> MGSS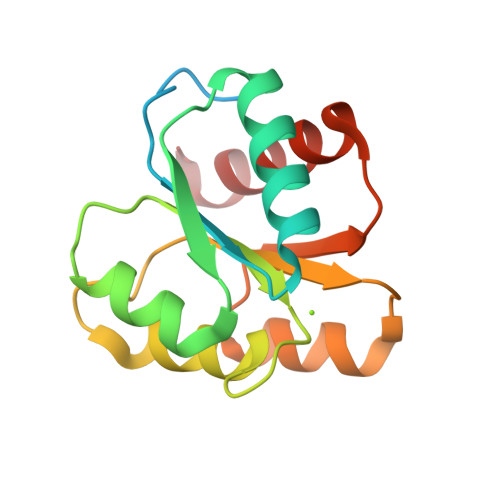HHHHHHSSGPQQGLRENLYFQGMADKELKFLVVDDFSTMRRIVRNLLKELGFNNVEEAEDGVDALNKLQAGGYGFVISDWNMPNMDGLELLKTIRADGAMSALPVLMVTAEAKKENIIAAAQAGASGYVVKPFTAATLEEKLNKIFEKLGM>GPLGSQLCGRVFKSGETTYSCRDCAIDPTCVLCMDCFQDSVHKNHRYKMHTS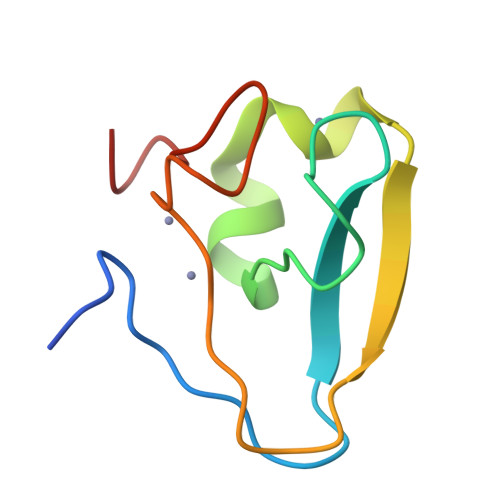TGGGFCDCGDTEAWKTGPFCVNHEP[2x]> AETCRIEAGDKQMTVNMGQISSNRFHAVGEDSAPVPFVIHLRECSTVVSERVGVAFHGVADGKNPDVLSVGEGPGIATNIG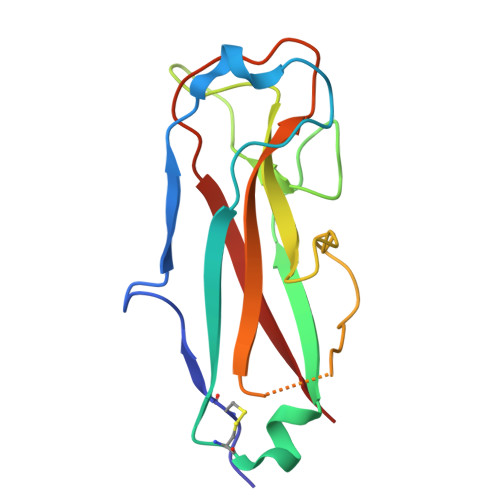VALFDDEGNLVPINRPPANWKRLYSGSTSLHFIAKYRATGRRVTGGIANAQAWFSLTYQ> MGSSHHHHHHSSNPAEGSPGPGTVFVYSGRGSQWAGMGRQLLADEPAFAAAVAELEPVFVEQAGFSLHDVLANGEELVGIEQIQLGLIGMQLALTELWCSYGVQPDLVIGHSMGEVAAAVVAGALTPAEGLRVTATRSRLMAPLSGQGGMALLELDAPTTEALIADFPQVTLGIYNSPRQTVIAGPTEQIDELITRVRARDRFASRVNIEVAPHNPAMDALQPAMRSELADLTPRTPTIGIISTTYADLHTQPVFDAEHWATNMRNPVHFQQAIASAGSGADGAYH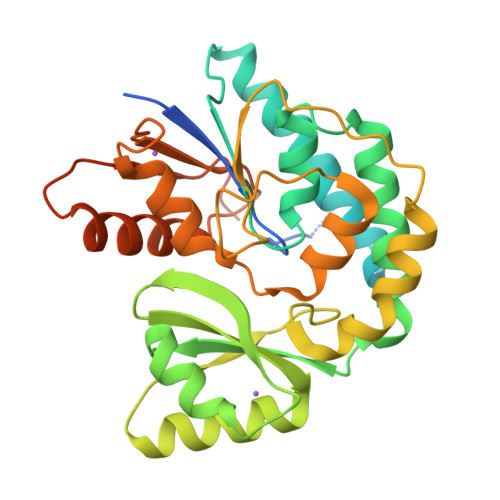TFIEISAHPLLTQAIIDTLHSAQPGARYTSLGTLQRDTDDVVTFRTNLNKAHTIHPPHGS>[5x]AQDMVSPPPPIADEPLTVNTGIYLIESYSLDDCAETFKVNAFLSLSWKDRRLAFDPVRSGVRVKTYEPEAIWIPEIRFVNVENARDADVVDISVSPDGTVQYLERFSARVLSPLDFRRYPFDSQTLHIYLIVRSVDTRNIVLAVDLEKVGKNDDVFLTGWDIESFTAVVKPANFALEDRLESKLDYQLRISRQYFS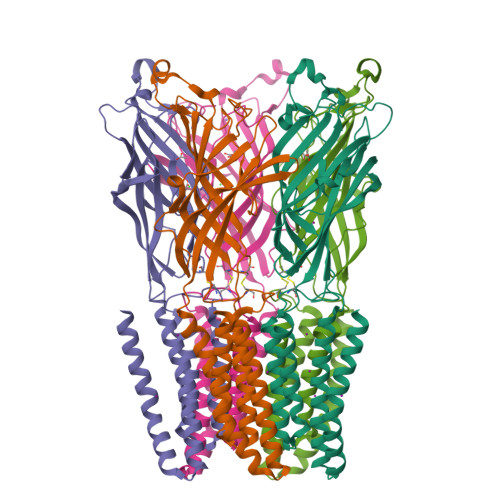YIPNIILPMLFILFISWTAFWSTSYEANVTLVVSTLIAHIAFNILVETNCPKTPYMTYTGAIIFMIYLFYFVAVIEVTVQHYLKVESQPARAASITRASRIAFPVVFLLANIILAFLFFGF(2~{R})-~{N}-[5-[3,5-bis(oxidanyl)phenyl]-4-ethanoyl-1,3-thiazol-2-yl]piperazine-2-carboxamide | C16 H18 N4 O4 S | 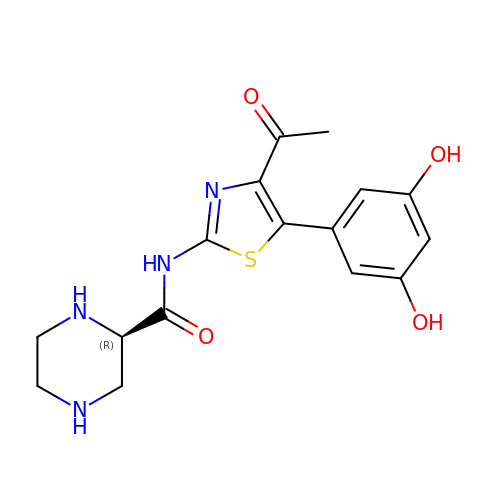XEVZKKXMSLWLTA-GFCCVEGCSA-N>MALAKRIDAALILKDGRVVKGSNFENLRDSGDPVELGKFYSEIGIDELSFWDITASVEKRKTMLELVEKVAEQIDIPITVGGGIYDFETASELILRGADKVEINTAAVENPSLITQIAQTFGSQAVVVYIAAKRVDGEFMVFTYSGTKNTGILLRDWVVEVEKRGAGEIVLGSIDRLGTKSGYDTEMIRFVRPLTTLPIIAHRGAGKTEHFLEAFLAGADAAKADSVFHSREIDVRELKEYLKKHGVNVRLEGLGSLEHHHHHH[2x]

Computational design of KE07 involved construction of a theozyme to catalyze the chemical reaction, which was then grafted into the scaffold of imidazole glycerol phosphate synthase (HisF) from Thermotoga maritima. Catalytically essential residues from the initial design include a base (Glu101) that facilitates C−H bond cleavage, an H-bond donor (Lys222) to stabilize the phenoxide intermediate, and a π-stacking residue (Trp50), which was designed to stabilize the transition state and favor substrate binding through interactions with the aromatic ring of the substrate. This initial KE07 design (Round 1; R1) catalyzes the cleavage of 5-nitrobenzisoxazole, with 103-fold rate acceleration over the noncatalyzed reaction and a turnover rate (kcat) of 0.018 s−1.

The mutations in R7 and R7-2 (Phe77Ile, Phe229Ser, Ile102Phe) result in further optimization of activation energy. For R7 and R7-2, we were able to capture the active site in configuration A when glycerol/Bis-Tris was used as cryoprotectant, and configuration B with the neighboring hexahistidine tag bound and MPD used as cryoprotectant. For example, Ile102Phe results in phenylalanine filling a hydrophobic cavity and a small adjustment of the main chain, which increases the distance between Glu101 and Trp50, allowing sampling of the Trp50 rotamer, which is then stabilized by an H-bond to Glu101, thereby stabilizing this alternative configuration. By R7 and R7-2, configuration C (which was the only state we saw associated with product in the crystal structures) becomes the dominant substate sampled, with configurations A and B sampled only rarely.> MSLTRRDFVKL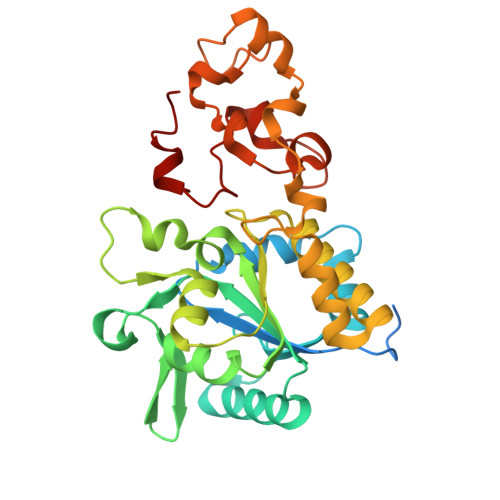CTGTVAGFGISQMFHPAVHEALAGTLTGERPPVFWLQGQGCTGCSVTLLNSVHPSIADVLLKVISLEFHPTVMAWEGEHAIEHMRKVAEKFKGKFFLVIEGSVPVEADGKYCIIGEANHHEISMVDALKEFGPNAAAVLAVGTCAAYGGIPAAEGSETGATAVSKFLGDNGIKTPVVNIPGCPPHPDWIVGTVVLALDAIKKNGLEGGLAEVVKVLDSDGRPTPFFGRNIHENCPYLDKYDEGVMSATFTDKVGCRYDLGCKGPMTMADCFERKWNGGVNWCVQNAVCIGCVEPDFPDGKSPFYQA> MSLAEVNPMSKPLVRWPINPLRTAVIVVDMQKVFCEPTGALYVKSTADIVQPIQKL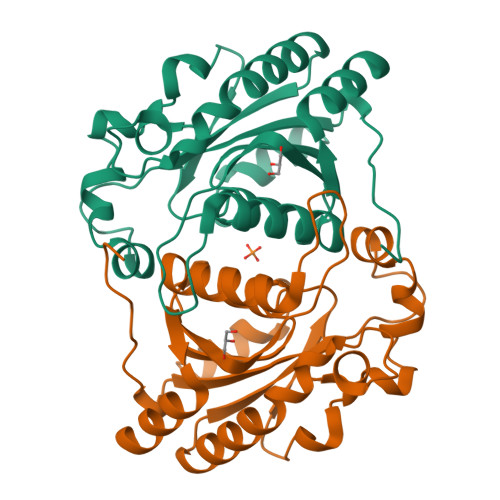LQAARAAQVMVIYLRHIVRGDGSDTGRMRDLYPNVDQILARHDPDVEVIEALAPQSDDVIVDKLFYSGFHNTDLDTVLRARDVDTIIVCGTVTNVCCETTIRDGVHREYKVIALSDANAAMDYPDVGFGAVSAADVQRISLTTIAYEFGEVTTTAEVIRRIESAYPHGREGHHHHHH> SATSLKQDADDMCMICFTEALSAAPAIQLDCSHIFHLQCCRRVLENRWLGPRITFGFISCPICKNKINHIVLKDLLDPIKELYEDVRRKALMRLEYEGLHKSEAITTPGVRFYNDPAGYAMNRYAYYVCYKCR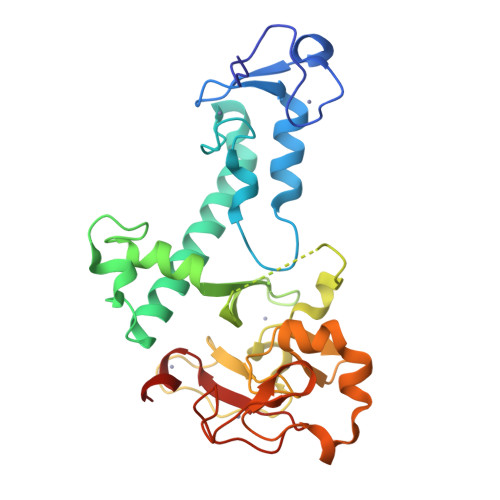KAYFGGEARCDAEAGRGDDYDPRELICGACSDVSRAQMCPKHGTDFLEYKCRYCCSVAVFFCFGTTHFCNACHDDFQRMTSIPKEELPHCPAGPKGKQLEGTECPLHVVHPPTGEEFALGCGVCRNAHTF> MGLFDRLGRVVRANLNDLVSKAEDPEKVLEQAVIDMQEDLVQLRQAVARTIAEEKRTEQRLNQDTQEAKKWEDRAKLALTNGEENLAREALARKKSLTDTAAAYQTQLAQQRTMSENLRRNLAALEAKISEAKTKKNMLQARAKAAKANAELQQTLAAAAAAAAAAAFERMENKVLDMEATSQAAGELAGFGIENQFAQLEASSGVEDELAALKASMAGGALPGTSAATPQLEAAPVDSSVPANNASQDDAVIDQELDDLRRRLNNLAALEVLFQGP

A prominent member of the PspA family is the vesicle-inducing protein in plastids 1 (Vipp1), also known as IM30 (inner membrane-associated protein of 30 kDa). Vesicle-inducing protein in plastids 1 (Vipp1) is critical for thylakoid membrane biogenesis and maintenance. Vipp1 appears to have two functions: in membrane maintenance (that is, during heat or light stress) and in thylakoid membrane (TM) biogenesis and/or remodeling. Vipp1 binds to negatively charged membranes and membrane binding depends on stored curvature elastic stress.

Moreover, by replacing the hinge 2 region of Vipp1 with ten alanines, we generated plasticity-restrained Vipp1 assemblies. The resulting variant Vipp1 dL10Ala indeed showed reduced structural plasticity when reconstituted with membranes, as it mostly formed type II tubes (69%), including single rings (27%) and stacked rings (3%), and type I tubes (2%). Therefore, we conclude that the mutated hinge 2 region is a critical element for the structural plasticity of Vipp1 assemblies. While we could reconstruct most of the structures formed by Vipp1 dL10 at low resolution, we could solve the structure of a subclass of type II tubes at 3.0-Å resolution, presumably because of the reduced flexibility. Outside of the different diameters and helical symmetries, the structures of both type II tubes were similar to the wild-type (WT) type II tubes with the monomers arranged approximately 45° to the tube axis. However, the dL10Ala monomer models had an overall extended length and showed less flexibility in the hinge 2 region, especially in single-ring monomers, which also explains the observed larger diameters of dL10Ala rings, as smaller rings require stronger bended and less extended monomers. The type II tubes have one continuous approximately 170-Å-long α-helix formed by α2, α3 and α4 presumably stabilized by the introduced deca-alanine stretch. The monomer structure of the type IIb tubes revealed another unique feature of this assembly, namely the fractured structure helix α5 that is split into two separate helices while still maintaining the canonical ESCRT-III α1−α3 hairpin-to-α5 contacts. The 3.0-Å-resolution structure of a plasticity-restrained Vipp1 dL10Ala mutant revealed the amphipathic positioning of helix α0 with the hydrophobic face directed into the tube lumen to potentially interact with hydrophobic acyl chains while the positive helix face interacts with the inner Vipp1 ring or tube surface and may be capable of interacting with lipid head groups. Our 3.0-Å Vipp1 tube structure now reveals that D5, R6, R9, R12 and E23 of α0 interact with three different subunits through α4 (R170), α4 (K174) and α1 (D35) to hold these helices in place, thereby aligning the interacting subunits and helices in an orientation favoring rings and type I and II tubes over the PspA-like assembly, in addition to described lipid interaction properties.> PPP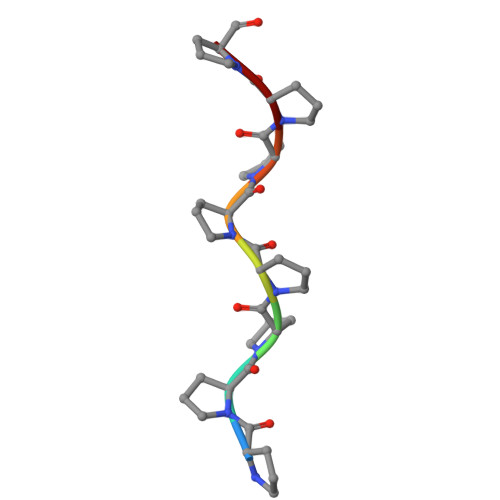PPPPP> YQDLRRRFFXHHLXAEXH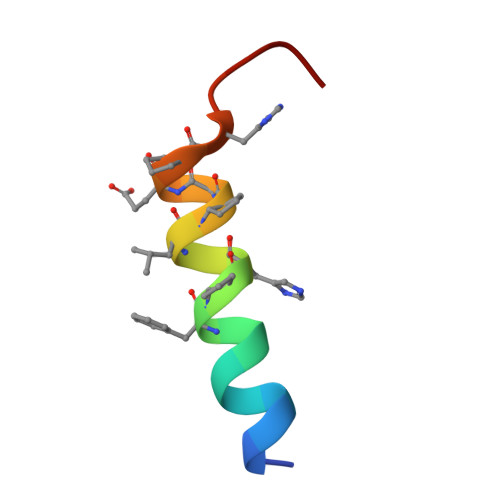TAEI TDO and IDO are heme proteins that catalyze the oxidative cleavage of L-Trp, the first and rate-limiting step of the kynurenine pathway for L-Trp catabolism. TDOs are homo-tetrameric enzymes with 35–45 kD monomers and are well conserved from bacteria to humans. The hTDO monomer has an all α-helical structure, and the helices are named αA through αL, as in XcTDO. The heme is located at one end of this four-helical bundle, with the proximal His328 ligand coming from the C-terminal region of helix αJ.

To define the binding mode of O2 with respect to L-Trp and to obtain direct molecular insight into the catalytic mechanism, we prepared crystals of ferrous hTDO in complex with L-Trp under anaerobic conditions and then exposed them to an O2-saturated solution at room temperature. In contrast, no electron density for O2 was observed in crystals mounted directly in the glove box, and the structure of hTDO in this binary complex with L-Trp is mostly the same as that obtained following O2 exposure. The recognition of the L-Trp substrate by hTDO is similar to that by XcTDO, as most of the residues in the active site region of the two enzymes are conserved. His76 is hydrogen-bonded to the N1 atom of L-Trp, although this interaction is not essential for TDO catalysis and this residue is replaced by Ser in IDO. The structure revealed that a second L-Trp molecule is bound to each hTDO subunit, with well-defined electron density. This exo site is located at the other end of the four-helical bundle and is ~42 Å from the active site. The side chain of this L-Trp is sandwiched between Trp208 (helix αH) and Pro213, and is in direct contact with several other hydrophobic residues. The main-chain carboxylate group has bidentate ion-pair interactions with the side chain of Arg211 (αH).

>MLPVEGSEEDKSQTGVNRASKGGLIYGNYLHLEKVLNAQELQSETKGNKIHDEHLFIITHQAYELWFKQILWELDSVREIFQNGHVRDERNMLKVVSRMHRVSVILKLLVQQFSILETMTALDFNDFREYLSPASGFQSLQFRLLENKIGVLQNMRVPYNRRHYRDNFKGEENELLLKSEQEKTLLELVEAWLERTPGLEPHGFNFWGKLEKNITRGLEEEFIRIQAKEESEEKEEQVAEFQKQKEVLLSLFDEKRHEHLLSKGERRLSYRALQGALMIYFYREEPRFQVPFQLLTSLMDIDSLMTKWRYNHVCMVHRMLGSKAGTGGSSGYHYLRSTVSDRYKVFVDLFNLSTYLIPRHWIPKMNPTIHKFLEHHHHHH[4x]>[2x]SRKTYTLTDYLKNTYRLKLYSLRWISDHEYLYKQENNILVFNAEYGNSSVFLENSTFDEFGHSINDYSISPDGQFILLEYNYVKQWRHSYTASYDIYDLNKRQLITEERIPNNTQWVTWSPVGHKLAYVWNNDIYVKIEPNLPSYRITWTGKEDIIYNGITDWVYEEEVFSAYSALWWSPNGTFLAYAQFNDTEVPLIEYSFYSDESLQYPKTVRVPYPKAGAVNPTVKFFVVNTDSLSSVTNATSIQITAPASMLIGDHYLCDVTWATQERISLQWLRRIQNYSVMDICDYDESSGRWNCLVARQHIEMSTTGWVGRFRPSEPHFTLDGNSFYKIISNEEGYRHICYFQIDKKDCTFITKGTWEVIGIEALTSDYLYYISNEYKGMPGGRNLYKIQLSDYTKVTCLSCELNPERCQYYSVSFSKEAKYYQLRCSGPGLPLYTLHSSVNDKGLRVLEDNSALDKMLQNVQMPSKKLDFIILNETK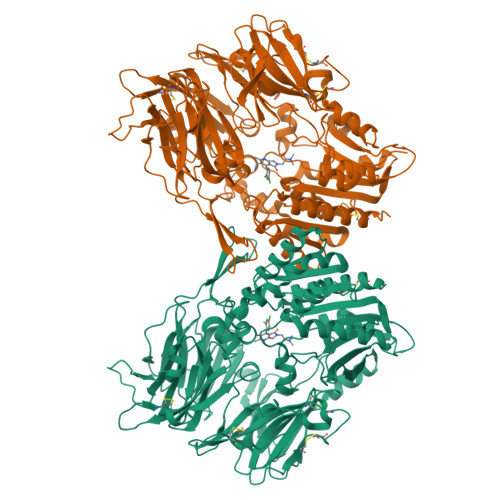FWYQMILPPHFDKSKKYPLLLDVYAGPCSQKADTVFRLNWATYLASTENIIVASFDGRGSGYQGDKIMHAINRRLGTFEVEDQIEAARQFSKMGFVDNKRIAIWGWSYGGYVTSMVLGSGSGVFKCGIAVAPVSRWEYYDSVYTERYMGLPTPEDNLDHYRNSTVMSRAENFKQVEYLLIHGTADDNVHFQQSAQISKALVDVGVDFQAMWYTDEDHGIASSTAHQHIYTHMSHFIKQCFSLP>[2x]MTVTTTYPGVYLSEDAVSSF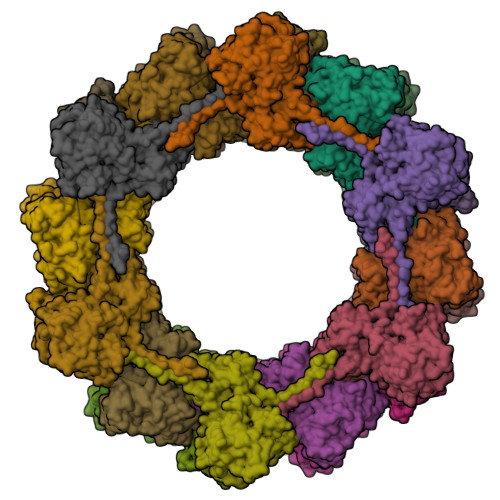SVNSAATAVPLFAYDSENTNTINKPIQVFRNWAEFTVEYPTPLEDAFYTSLSLWFMHGGGKCYLVNEANIADAVAQYDDITLIVAAGTDTTTYTAFTTVVGQGYRIFGLFDGPKEKIAGTAKPDEVMEEYPTSPFGAVFYPWGTLASGAAVPPSAIAAASITQTDRTRGVWKAPANQAVNGVTPAFAVSDDFQGKYNQGKALNMIRTFSGQGTVVWGARTLEDSDNWRYIPVRRLFNAVERDIQKSLNKLVFEPNSQPTWQRVKAAVDSYLHSLWQQGALAGNTPADAWFVQVGKDLTMTQEEINQGKMIIKIGLAAVRPAEFIILQFSQDIAQ;> MATVTSVPGVYIEEDASPAMSVSASATAVPLFVARFTPLKPELAGVITRIGSWLDYTILFDSNVPSSARVTVSSTAVEPSPEFDALETASSKATTTYTYQIDDTEVVDPTASVALRLYFQNGGGPCYLYPLEKADDNGPLAALPDLIDEVGEITLLASPDPDETYRTAVYGALAASLDQHKGYFLLADSVNGDAPSAVGGSAQVAVYYPNVEVPHTRKLDDAEVAIDGYLDDEGKAVTTLAALRVVNTEFAGEIAQSLSGDLSAPLSLPPSALIAGVYGKTDGERGVWKAPANVVLNGVSDVSVRVTNEQQAELNPKGINVIRHFSDRGLVVWGSRTQKDDDDWRYIPVRRLFDAAERDIKKALQPMVFEPNSQLTWKRVQTAIDNYLYRLWQQGALAGNKAEEAYFVRVGKGITMTQDEINQGKMIIQVGMAAVRPAEFIILKFTQDMSQ;> MTMVLPGVSYNETLLTQASNDDPVTMPLFIGYTPPDTAIPVTVMQPVSVGSLTQANSLFGQRGTLAYSLRHFFENGGLQCYVLPLGPGKGEPAARLQELIAALQTPQMLETLLADDKTGLVLVPELSELNEVSSTSLSAEGVDAAEVDADALWYQGWQVLLTLCRQAPQRFALLELPEDPASAVTLTQQSFSADQCQRGAAWWPRLETSYQDESSAPVVLSPLPAVAAAIQRSAHDNGVWKAPANIALAKTRRPTQSILTSQALLDNQGVSCNLIRSFVGKGVRLWGCRTLLNEENTAWRYIQIRLLVSSVEHYLSKLARAYLFEPNTAPTWMKLKGQVWTWLRQQWLAGAFFGTVEDEAFSLSIGLDETMTEDDIRHGKMILQVRLALLAPAEFIAISLTLDLRDGTASAQTGGQS> 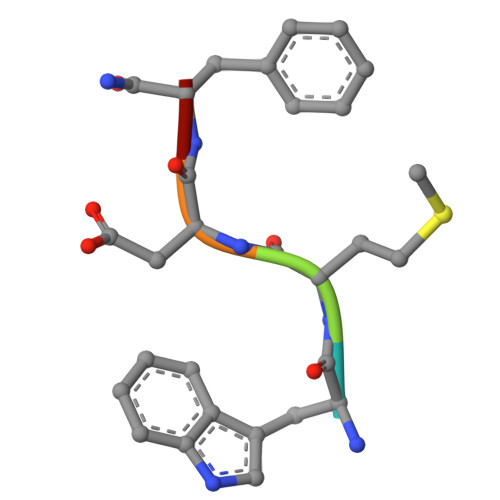WMDFX> MATVTATTKVPEIRDVTRIERIGAHSHIRGLGLDDALEPRQASQGMVGQLAARRAAGVVLEMIREGKIAGRAVLIAGQPGTGKTAIAMGMAQALGPDTPFTAIAGSEIFSLEMSKTEALTQAFRRSIGVRIKEETEIIEGEVVEIQIDRPATGTGSKVGKLTLKTTEMETIYDLGTKMIESLTKDKVQAGDVITIDKATGKISKLGRSFTRARDYDAMGSQTKFVQCPDGELQKRKEVVHTVSLHEIDVINSRTQGFLALFSGDTGEIKSEVREQINAKVAEWREEGKAEIIPGVLFIDEVHMLDIESFSFLNRALESDMAPVLIMATNRGITRIRGTSYQSPHGIPIDLLDRLLIVSTTPYSEKDTKQILRIRCEEEDVEMSEDAYTVLTRIGLETSLRYAIQLITAASLVCRKRKGTEVQVDDIKRVYSLFLDESRSTQYMKEYQDAFLFNELKGETMDTS

RuvB-Like (RuvBL) proteins are found in the domains Archaea and Eukarya, including humans and fungi, where they exert roles in transcription regulation, DNA damage repair, cell cycle control, stress adaptation and disease. The RuvB-Like family includes two homologous members, RuvBL1 and RuvBL2. As constituents of chromatin remodeling machines, RuvBL1 and RuvBL2 are involved in epigenetic regulation of transcription through the deposition of H2A.Z in nucleosomes flanking nucleosome-depleted regions around promoters (SWR1), by remodeling nucleosomes in order to increase DNA accessibility for the transcription and repair machinery, by enabling progression of stalled replication forks (INO80) and by the acetylation of histones H2A and H4, increasing chromatin accessibility (TIP60). The RuvBL1/2 complex functions as chaperone itself during the biogenesis of Telomerase, H/ACA RNPs and other supramolecular complexes.

The crystal structure of the full-length human transcription regulation factor RuvB-Like 2 (hsRuvBL2) in its apo form was determined to 2.89 Å resolution. The structure shows a hexameric arrangement of monomers similar to other structures in the RuvB-Like family. In the ring-shaped hsRuvBL2 hexamer, each protomer comprises the typical Rossman-like αβα fold (domain I) and the canonical all-α subdomain (domain III), which form the ATPase core together with the internal region of domain II. Moreover, there is an outward-facing mobile unit composing the external region of domain II, linked to the ATPase core by two β-sheet linkers. This unit is absent in all previous crystal structures of human RuvBL2 and is observed here for the first time. The interfaces between protomers form a complete nucleotide binding pocket, which includes the canonical nucleotide-binding motifs in domains I and III: Walker A (G77-T84), Walker B (D299-H302), sensor 1 (M326-N329), sensor 2 (T397-A402) and a trans-arginine finger (R353) from the adjacent protomer. Despite the fact that all purification steps were performed in the presence of ADP, no electron density corresponding to this nucleotide (or segments thereof), could be observed in the pocket. In addition to the overall mobility of domain II, there are four additional loops that are probably too mobile to produce an electron density: D148 - G159, D185 - V187, S203 - C227 and R253 - Q255. Thus, our apo hsRuvBL2 structure provides a missing link that supports the mechanism proposal whereby the N-terminal loop provides an interface between the external region of domain II and the ATPase core.Pum is a founding member of the Pum/fem-3 mRNA-binding factor (FBF), or PUF family, of eukaryotic RBPs. Pum binds with high affinity to specific sequences in target mRNAs and represses protein expression and enhances mRNA degradation. Regulation of hb mRNA by Pum relies on the spatial distribution of Nos, a tandem CCHC Zn finger (ZF) RBP. Here, we report the crystal structures of Nos-Pum-RNA complexes, which reveal that Nos acts as a molecular clamp that embraces both Pum and RNA.

We also determined a 1.14 Å crystal structure of a binary complex of Pum and a hb PRE2 RNA (5´-UGUACAUA), which exemplifies the modular 1 repeat:1 RNA base recognition of classical PUF proteins. For example, the UGU motif of the PRE is recognized by repeats R8 through R6. While the overall structure of Pum in the ternary complex is similar to that in the binary complex (RMSD of 1.2 Å over 324 Pum Cα atoms), the C-terminal region of Pum undergoes notable changes. Since the upstream nucleotides were not present in the binary complex, the change in the structure of the C-terminal region of Pum may be induced by the presence of the upstream RNA and/or Nos. With these conformational changes, Pum and Nos interact with one another and together recognize RNA immediately 5´ of the core PRE motif. Pum binds to the hb PRE2 using the base-omission mode observed for human Pumilio1, where bases +4 and +5 stack directly. Pum binds specifically to the 3´ AUA sequence at positions +6 to +8 of hb PRE2 RNA.

> SGRSRLLEDFRNQRYPNLQLRDLANHIVEFSQDQHGSRFIQQKLERATAAEKQMVFSEILAAAYSLMTDVFGNYVIQKFFEFGTPEQKNTLGMQVKGHVLQLALQMYGCRVIQKALESISPEQQQEIVHELDGHVLKCVKDQNGNHVVQKCIECVDPVALQFIINAFKGQVYSLSTHPYGCRVIQRILEHCTAEQTTPILDELHEHTEQLIQDQYGNYVIQHVLEHGKQEDKSILINSVRGKVLVLSQHKFASNVVEKCVTHATRGERTGLIDEVCTFNDNALHVMMKDQYANYVVQKMIDVSEPTQLKKLMTKIRPHMAALRKYTYGKHINAKLEK> GTEDLYFQSHMTIAVTGSIATDHLMRFPGRFSEQLLPEHLHKVSLSFLVDDLVMHRGGVAGNMAFAIGVLGGEVALVGAAGADFADYRDWLKARGVNCDHVLISETAHTARFTCTTDVDMAQIASFYPGAMSEARNIKLADVVSAIGKPELVIIGANDPEAMFLHTEECRKLGLAFAADPSQQLARLSGEEIRRLVNG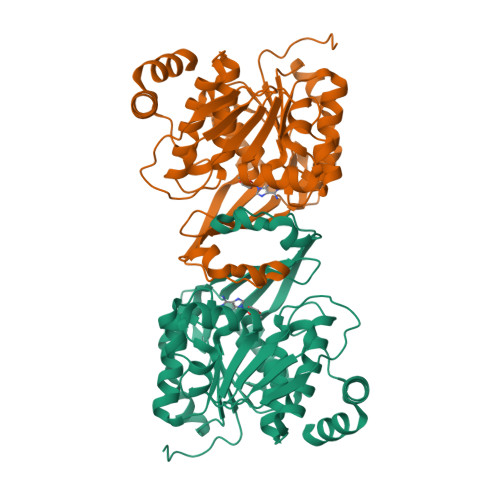AAYLFTNDYEWDLLLSKTGWSEADVMAQIDLRVTTLGPKGVDLVEPDGTTIHVGVVPETSQTDPTGVGDAFRAGFLTGRSAGLGLERSAQLGSLVAVLVLESTGTQEWQWDYEAAASRLAGAYGEHAAAEIVAVLA>SMADVSLFFGGLPAILLKADTIYRIGRQKGLEISIADESMELAHATACILRRGVVRLAALVGKI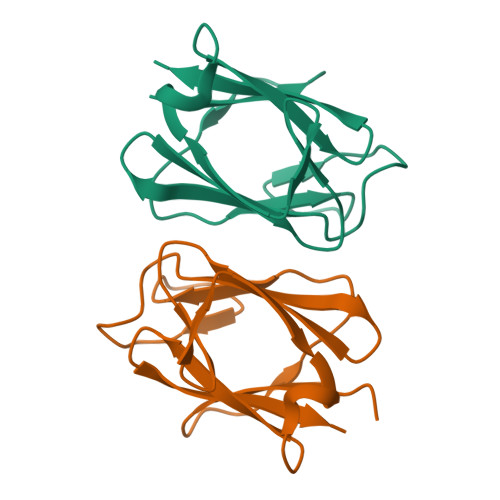FVNDQEETVVDIGMENAVAGKVKLRFGNVEARLEFGED[2x]>AKALEQPFDVANIPGPKMATLLEKGKPVANMIKKAKRPLLIVGPDMTDEMFERVKKFVEKDITVVATGSAITRFIDAGLGEKVNYAVLHELTQFLLDPDWKGFDGQGNYDLVLMLGSIYYHGSQMLAA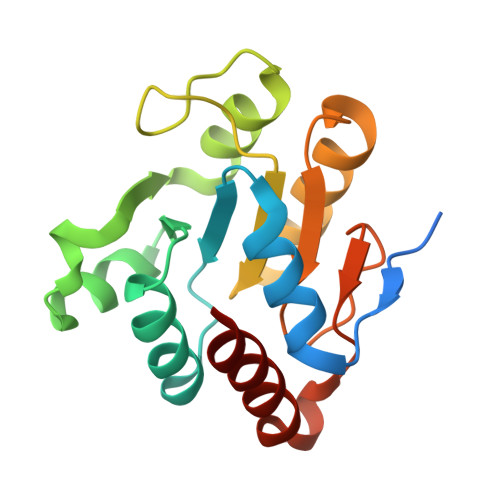IKNFAPHIRALAIDRYYHPNADMSFGNLWKKEEDYLKLLDEILAEL[4x]> MSLTAIHRPTWVSVDLDAAAHNLQEIREWTKAKKVYAVLKADGYGLGAIPLAKAFQETASADALIVSNLDEALELRQADLTLPIWVLGAWDYSDLKLFIDHD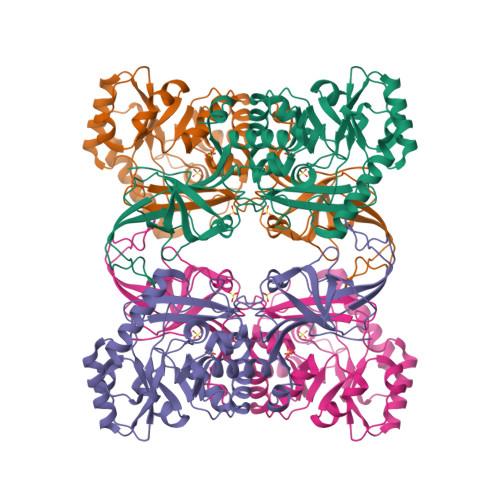IVITIPSLAWLQNLPDFEGTLKVSLAIDTGMTRIGFDKADEISAAKKIIDKNPQLDLFSVYTHFATADEAGEKSKAYFEEQLRRWQELTINQGFDPSLFSMANSATCIWHHDDPRISFAAIRPGQLISGVNVSNGELKMPPNLHLERIFSVCSEIADVRFVKKDQSLSYGASERMPEDGYVATLPFGYNDGWLRRMQKSSVIINGKRMPIIGRITMDQTMVKLDRKYPIGTRVTLIGKDGGEQITVEEVANYSHTIVDEIQTTLAPRIKRIYTGDLAEVIGANYGEGHHHHHH> MGGVAMPGAEDDVVRENLYFQGKDGLAAMENA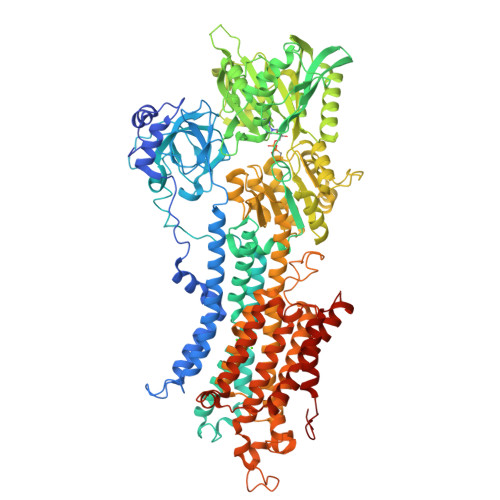HTKTVEEVLGHFGVNESTGLSLEQVKKLKERWGSNELPAEEGKTLLELVIEQFEDLLVRILLLAACISFVLAWFEEGEETITAFVEPFVILLILVANAIVGVWQERNAENAIEALKEYEPEMGKVYRQDRKSVQRIKAKDIVPGDIVEIAVGDKVPADIRLTSIKSTTLRVDQSILTGESVSVIKHTDPVPDPRAVNQDKKNMLFSGTNIAAGKAMGVVVATGVNTEIGKIRDEMVATEQERTPLQQKLDEFGEQLSKVISLICIAVWIINIGHFNDPVHGGSWIRGAIYYFKIAVALAVAAIPEGLPAVITTCLALGTRRMAKKNAIVRSLPSVETLGCTSVICSDKTGTLTTNQMSVCRMFILDRVEGDTCSLNEFTITGSTYAPIGEVHKDDKPVNCHQYDGLVELATICALCNDSALDYNEAKGVYEKVGEATETALTCLVEKMNVFDTELKGLSKIERANACNSVIKQLMKKEFTLEFSRDRKSMSVYCTPNKPSRTSMSKMFVKGAPEGVIDRCTHIRVGSTKVPMTSGVKQKIMSVIREWGSGSDTLRCLALATHDNPLRREEMHLEDSANFIKYETNLTFVGCVGMLDPPRIEVASSVKLCRQAGIRVIMITGDNKGTAVAICRRIGIFGQDEDVTSKAFTGREFDELNPSAQRDACLNARCFARVEPSHKSKIVEFLQSFDEITAMTGDGVNDAPALKKAEIGIAMGSGTAVAKTASEMVLADDNFSTIVAAVEEGRAIYNNMKQFIRYLISSNVGEVVCIFLTAALGFPEALIPVQLLWVNLVTDGLPATALGFNPPDLDIMNKPPRNPKEPLISGWLFFRYLAIGCYVGAATVGAAAWWFIAADGGPRVSFYQLSHFLQCKEDNPDFEGVDCAIFESPYPMTMALSVLVTIEMCNALNSLSENQSLLRMPPWENIWLVGSICLSMSLHFLILYVEPLPLIFQITPLNVTQWLMVLKISLPVILMDETLKFVARNYLEPGKECVQPATKSCSFSACTDGISWPFVLLIMPLVIWVYSTDTNFSDMFWS We have utilised the prokaryotic Kir channel KirBac3.1 to determine whether the acyl tails of bound lipids, protruding into the conduction pathway through fenestrations just below the selectivity filter, might represent key gating elements. In KirBac3.1, the four Leu124 residues form a steric cluster physically occluding the conduction pathway, separating the cavity into upper and lower vestibules, while Tyr132 (at the inner helix bundle) forms a non-occlusive hourglass-shaped portal between lower vestibule and cytosol. Here we present evidence that in Kir channels, a limiting barrier to permeation within the conduction pathway is formed by a collar of branched aliphatic side chains. We show that acyl tails of tightly bound lipids occupying conserved fenestrations into the pore engage individual side chains of the collar, drawing them away from the central conduction pathway and allowing ions to pass.

Reasoning that the chemistry of the contributing side chains determines their mutual affinity and propensity to form a steric barrier, we mutated the branched aliphatic residue Leu124 to the linear methionine, which is similar in both molecular volume and hydrophobicity, but more flexible. Conversely, L124M assays showed enhanced channel activity, significantly outperforming KirBac3.1 in the fluorometric assay. We determined a crystal structure of L124M in case the increased activity was due to structural distortion (such as forcing the inner helices apart). The mutation was made on a background in which two native cysteines were mutated to serine (C71S-C262S; SCS) and thus we also determined a structure of the KirBac3.1-SCS background crystallised under the same conditions. We also carried out single-channel recordings of the reconstituted L124M channels in lipid bilayers, revealing currents exhibiting the sub-conductance states typifying KirBac3.113. We also carried out simulations on the L124M mutant, using the crystal structure as a starting model, finding a negligible barrier to K+ permeation at the collar. We reasoned that if the leucine collar is the primary permeation gate and the role of the lipid tails is to competitively displace individual leucine side chains, thereby compromising the collar, lipids should not be required for permeation in the L124M mutant with its labile methionine sidechains. Indeed, L124M with all four Tyr57 adopting gauche rotamers appeared as effective at conducting K+ as wild type KirBac3.1 with all Tyr57 side chains trans, indicating that the interaction with aliphatic lipid tails in wild type is only required because of the inflexible steric occlusion created by Leu124 residues. In simulations, the L124M mutant was able to conduct even when lipid tails were prevented from entering fenestrations, demonstrating the unbranched aliphatic residue methionine does not form a significant barrier to permeation; L124M is essentially ungated.

> MTGGMKPPARKPRILNSDGSSNITRLGLEKRGWLDDHYHDLLTVSWPVFITLITGLYLVTNALFALAYLASGDVIENARPGSFTDAFFFSVQTMATIGYGKLIPIGPLANTLVTLEALCGMLGMAVAASLIYARFTRPTAGVLFSSRMVISDFEGKPTLMMRLANLRIEQIIEADVHLVLVRSEISQEGMVFRRFHDLTLTRSRSPIFSLSWTVMHPIDHHSPIYGETDETLRNSHSEFLVLFTGHHEAFAQNVHARHAYSSDEIIWGGHFVDVFTTLPDGRRALDLGKFHEIAQHHHHHH(3S)-1-[(2S)-2-methyl-3-sulfanyl-propanoyl]piperidine-3-carboxylic 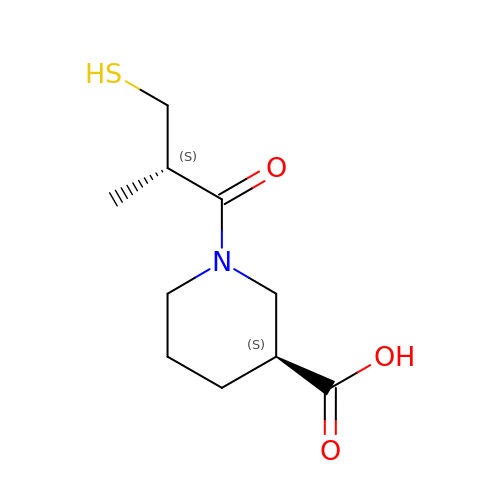acid | C10 H17 N O3 S | DZPFHBBJBWEEDM-SFYZADRCSA-N> RLVDTDGK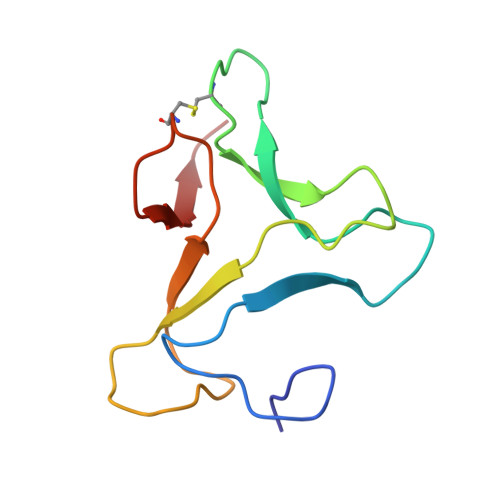PIENDGAEYYILPSVRGKGGGLVLAKSGGEKCPLSVVQSPSELSNGLPVRFKASPRSKYISVGMLLGIEVIESPECAPKPSMWSVKSG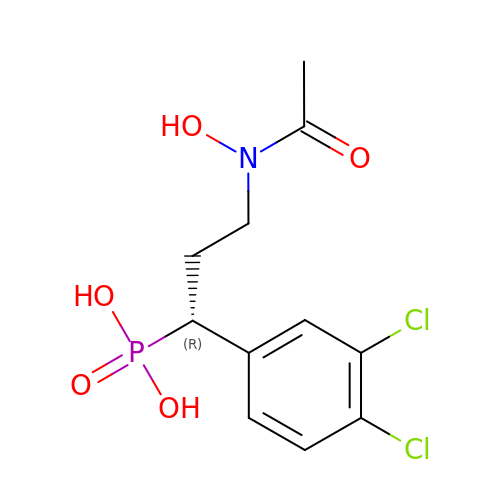[(1R)-3-[acetyl(hydroxy)amino]-1-(3,4-dichlorophenyl)propyl]phosphonic acid | C11 H14 Cl2 N O5 P | ABGCTQYLJZGMBM-LLVKDONJSA-N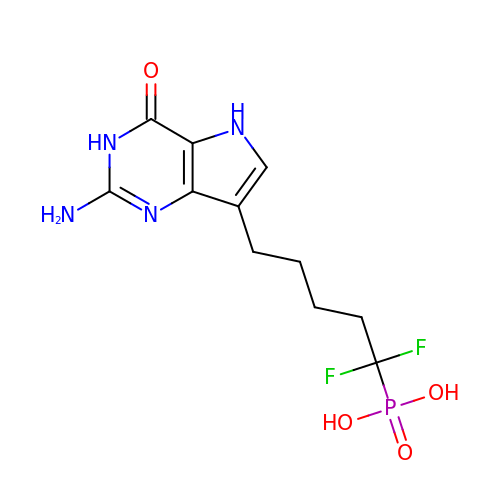[5-(2-amino-4-oxo-4,5-dihydro-3H-pyrrolo[3,2-d]pyrimidin-7-yl)-1,1-difluoropentyl]phosphonic acid | C11 H15 F2 N4 O4 P | OISKFAFOKMNXNK-UHFFFAOYSA-N>[2x]SNAMTPETNETLKLIGSDKVQGTAVYGPDGEKIGSIERVMIE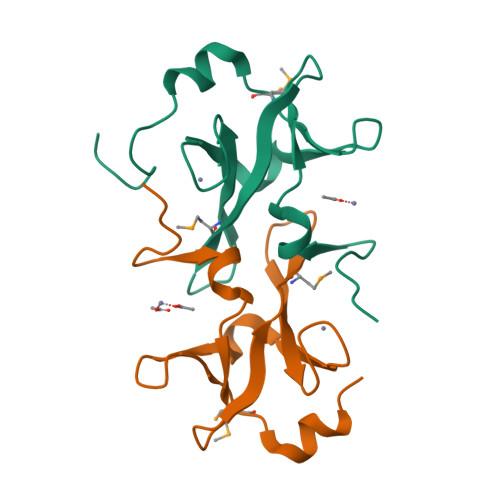KVSGRVSYAVLSFGGFLGIGDDHYPLPWPALKYNVELGGYQVMVTVDQLERAPKYGPGSEWDWRGARKVDDYYGVALT>QNSLALH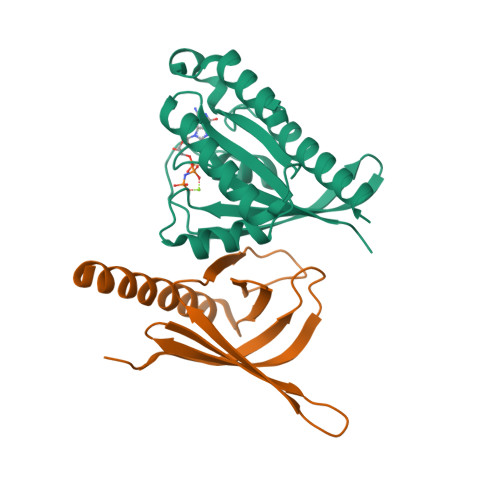KVIMVGSGGVGKSALTLQFMYDEFVEDYEPTKADSYRKKVVLDGEEVQIDILDTAGLEDYAAIRDNYFRSGEGFLCVFSITEMESFAATADFREQILRVKEDENVPFLLVGNKSDLEDKRQVSVEEAKNRAEQWNVNYVETSAKTRANVDKVFFDLMREIRARKMEDS[2x];>LETPGQYLVYNGDLVEYEADHMAQLQRVHGFLMNDCLLVATWLPQRRGMYRYNALYPLDRLAVVNVKDNPPMKDMFKLLMFPESRIFQAENAKIKREWLEVLEETKRALSDKRRREQEEA[2x]>MSLSAMPAALSFAGLAGWAEEDHLAALNAFRAGCGVSKDPAAARVCGLAKATKDLDVSGAKAFIEANFRVEAVDGGGDGLLTAYFAPQYEARMSRNAEFSAPLRGLPADLVVLDLGPFEPALVGKKITGHVEGSTFVPYPDRAEIEATPSDKPLAWMRPEELFFLQIQGSGVLVLPDGRRVRAVFAGTNGKPFVGIAIAMRDKGLLPDNNTSADAIRTWLAEHRGPEADAIMRLNPRYVFFRTVPDDGKEPAGAAGVALPPGRAIAVDPGYHAYGGF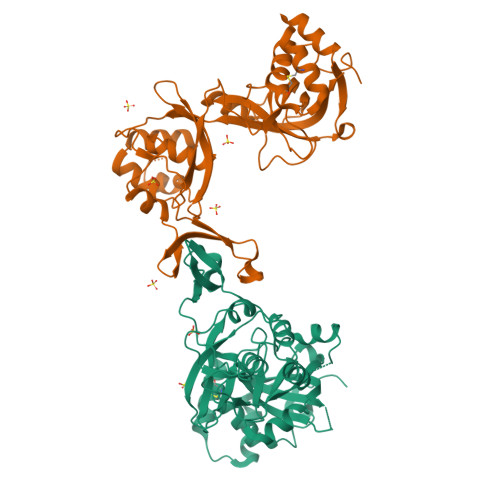YWLDAAAPKLVGAFPVYRRAVTALDTGGAIKGEVRADLYMGSGAVAGVEAGRVRHTLRLYRLTPNPEGHHHHHH[2x]>MYNDDYIEEASFLNGSDVVILIDGVEELYMEEIKADFEQDEQSIKLLGCQNEISRVGTTKGSFSLNGYKTDSKFAKLGFRSFEIIYNLSNSETLGYESIRLKNCRLKKLPLINSKAGEIVKIEVEGSFRGYDLLNEL[6x];>MINIDRRRKDIIRTININPTNITITSIKKTEIDGAFEETETEIKCVVRIFNEKTAEKQISSEKQGTFSSIRTYGMLVSNDVILEVNSRDSLEFECIYGRMKIVNIYPQIVKGELCGYQCSLERID[6x];>MRAGIRKALIDNIKELKGCYEPNVPNKDTKKPYMVVVQGQDNDHGETIGFERSIEVWIYEGRTTFKKLDKLTKQVVEVLDMNTIVDESENEAFTCIYKGTSENDIVVEEWDAIARGIRFSVIALEDKEDTTNDRWVEALSRHTKDLLEIESYKDNWKKNFIAPCALWRTTHIENKRINYHLIEITKTMKCHVVSKNKDEIVKLLETLETSLIIDKRVRLREDKNMYLTLVSVVEDRESDMFTTGQLTAVFKMIGKIKREGPTMDKIYGNGNLK[6x];>MTPARDLIEKLRLLLNDKDKKSFTDEELNLFLEEADCIYCAASQGWILKSLQYENTVGEMYEYKVGQETYKSSSIKDLVSVAYQNADKFKDMCTNKKEKGSFMLGISTEFEI[12x];>[6x]MATGTWNEKERKEIPGFYNRFKTQAEKSTNTGLKGRLAMPIRANWGDVGKVVTIKNDLRQLKNLFGDDMNYSAFKLGKLALLGNVKELLLYRLVDGNQKKGTLTLKDTTENSAKDVIKLETKYPTARNFNVTIKSNLVDSDKKDFIFFENTKQLFSSSIKGTIDEIVLEINSNLDNEYVIATKVADSDTILANVVNQALEGGNDGCTSITNESYLKALEEFERYSFDSFVLDGVADEALQETTKAWVAKNKELGKDILLFLGGKTEDNIKQINDKSKSFNDENIVNVGSSAYYENIKYTPSEVAVYIAALSVSKGITGSICNAKTIFEEVEPRLSQSEVKECLKSGTLVLDFDDGDVIIVDDVNTFKKYVDDKNEAMGYISNIMFINTINKDTSLKRKEFVGKIFNDATGQTTVICALKKYFEELMSQGIISEFNVDIDTELQATAKADEFYWKWDAVKVDVMKKIYGTGYLG;>[12x]MGIISYVKKLFKRPAGEIMRMSSGNIGVYKLDDSRVDYELARELYQNKNANYKLGSSFVRPIVNSTTGFMGVPHFQIEDEEAQYILDEFVLDNTSKMLKTHTDSLKQGDCYIWITREERENPLYPDKKVRLIYNFISPEEVKEIILDPTTKEPIAYILESQNEWTDLGENKRKAKVKQIITAESRFVEVEGDKIEGLEEGETPNVWGF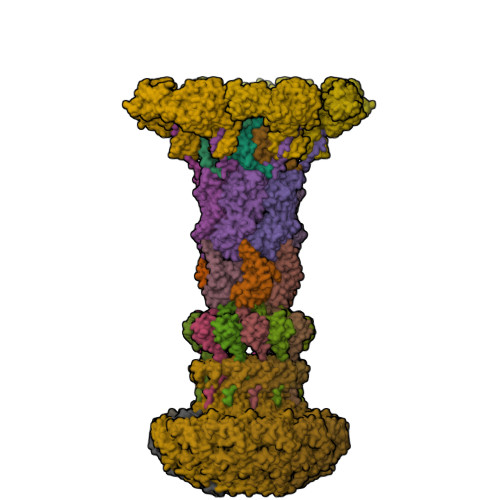IPIIHFKNEADETLKYGQSDIEPIEPLLKAYHDVMLHALKGSKMHSTPKLKLKLTDVASFLAHNFGVEDPVKFAKEGGKINLDGHEILFLNKDEEAEFVEVKSAIGDAKELLKLLFYCIVDVSETPEFIFGVHTPSALASVKEQMPIMVNKIRRKREQFTNSWQLLARMVLIMSSNSSGMKYSSYDVTIGWDEVNPRDDKELAETLEKVCCALDKALEGGFISEESTVNFLAQYIDTMSNYISDDPEREGEREKIIKTKMLKYRLDDSQGLNDESNEIEKEINKIKDNNGNG>[3x]AQVLRGTVTDFPGFDERADAETLRKAMKGLGTDEESILTLLTSRSNAQRQEISAAFKTLFGRDLLDDLKSELTGKFEKLIVALMKPSRLYDAYELKHALKGAGTNEKVLTEIIASRTPEELRAIKQVYEEEYGSSLEDDVVGDTSGYYQRMLVVLLQANRDPDAGIDEAQVEQDAQALFQAGELKWGTDEEKFITIFGTRSVSHLRKVFDKYMTISGFQIEETIDRETSGNLEQLLLAVVKSIR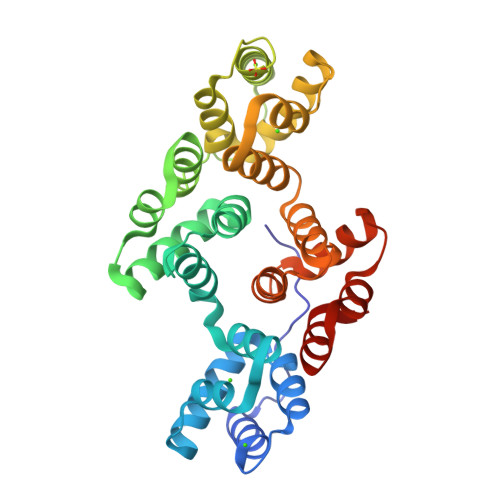SIPAYLAETLYYAMKGAGTDDHTLIRVMVSRSEIDLFNIRKEFRKNFATSLYSMIKGDTSGDYKKALLLLCGEDD>[2x]MKRFLLGLVLLLAVAAGVLYFVPATLLASVRTVERGLAGLSEHSVQVDNLEIAYLEGGSEKNPTLLLIHGFGADKDNWLRFARPLTERYHVVALDLPGFGDSS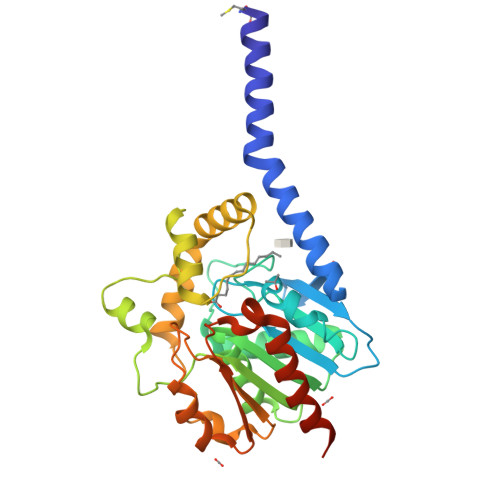KPQQASYDVGTQAERVANFAAAIGVRRLHLAGNSMGGHIAALYAARHPEQVLSLALIDNAGVMPARKSELFEDLERGENPLVVRQPEDFQKLLDFVFVQQPPLPAPLKRYLGERAVAASAFNAQIFEQLRQRYIPLEPELPKIEAPTLLLWGDRDRVLDVSSIEVMRPLLKRPSVVIMENCGHVPMVERPEETAQHYQAFLDGVRNAQVAGRGHHHHHH> NDDENERSRQIDDILEKTYYNVDTHPAESLDWFNVLIGQTIQQLREEAWKKDNIVYSLNAFIERKAQELPSYLDSIKITELDIGHDFPIFSNCRIQYSPNSNGRKLEAKIDIDLNDRLAVGIETRLLLNYPKPLTASLPINVTVSIIRFQACLTVSLTKAEEFVPT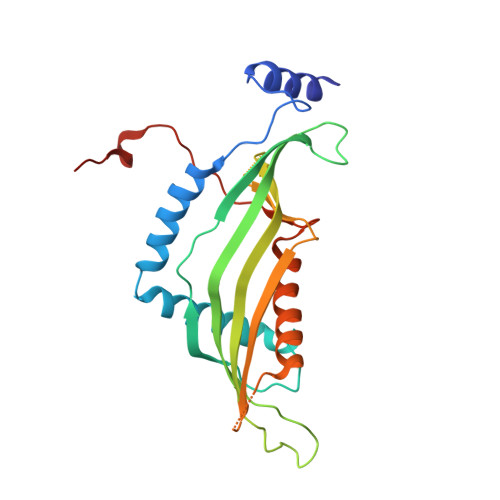SPESVDEDDNDGYFLMFSFAPEYRMEFETQSLIGARSKLENIPKIGSLVEYQIKKWFVERCVEPRFQFIKLPSVWPRSKNTREGKADVD>GPGSMTKTWTLKKHFVGYPTNSDFELKTSELPPLKNGEVLLEALFLTVDPYMRVAAKRLKEGDTMMGQQVAKVVESKNVALPKGTIVLASPGWTTHSISDGKDLEKLLTEWPDTIPLSLALGTVGMPGLTAYFGLLEICGVKGGETVMVNAAAGAVGSVVGQIAK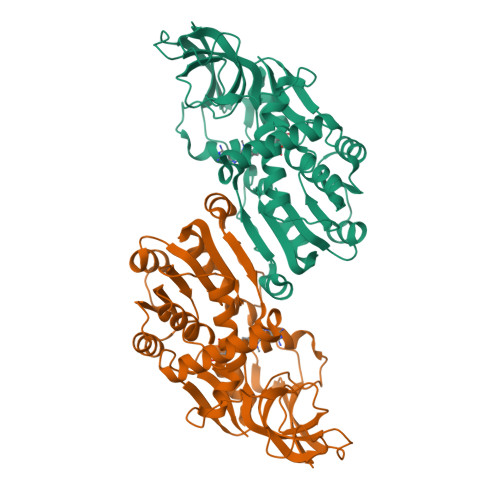LKGCKVVGAVGSDEKVAYLQKLGFDVVFNYKTVESLEETLKKASPDGYDCYFDNVGGEFSNTVIGQMKKFGRIAICGAISTYNRTGPLPPGPPPEIVIYQELRMEAFVVYRWQGDARQKALKDLLKWVLEGKIQYKEYIIEGFENMPAAFMGMLKGDNLGKTIVKA[4x]>[2x]GSGMMRYLHKIELELNRLTSRYPFFKKIAFDAEIIKLVDDLNVDENVKCAIVAIDTSMRMQDFINEDNKDSFVLSTDVLSALFYKYLSQPFYQHDFLVLTDCVSRINELKSIRATITDEIALHNINKQIHYMFIQPYMNNEKVVSYE;>MIALSYKAFLNPYIIEVEKRLYECIQSDSETINKAAHHILSSGGKRVRPMFVLLSGF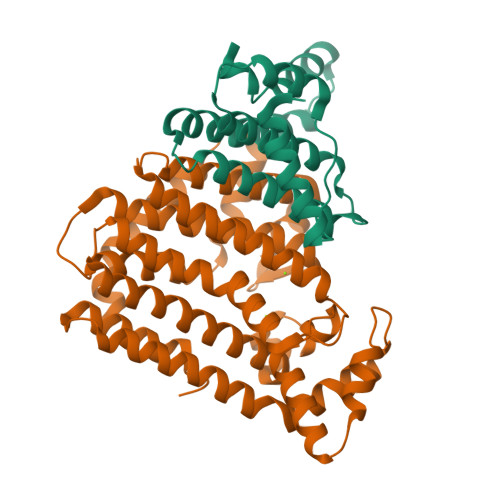LNDTQKDDLIRTAVSLELVHMASLVHDDYIDNSDMRRGNTSVHIAFDKDTAIRTGHFLLARALQNIATINNSKFHQIFSKTILEVCFGEFDQMADRFNYPVSFTAYLRRINRKTAILIEASCHLGALSSQLDEQSTYHIKQFGHCIGMSYQIIDDILDYTSDEATLGKPVGSDIRNGHITYPLMAAIANLKEQDDDKLEAVVKHLTSTSDDEVYQYIVSQVKQYGIEPAELLSRKYGDKAKYHLSQLQDSNIKDYLEEIHEKMLKRVY[2x]(4S)-2-(2-hydroxyphenyl)-4,5-dihydro-1,3-thiazole-4-carboxylic acid 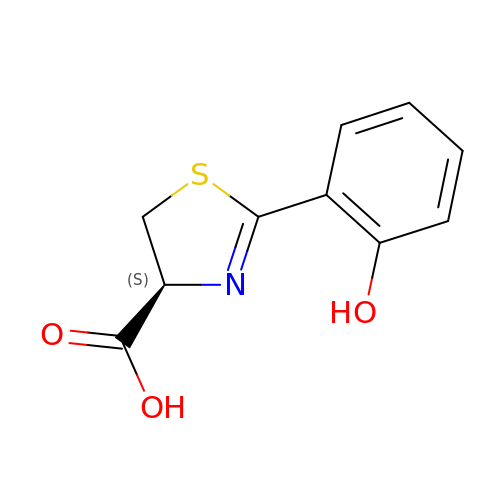| C10 H9 N O3 S | CECDPVOEINSAQG-SSDOTTSWSA-N>GSMPLLLDDGDPKAQTGFDLSTATTLFWRPVPVHVKQQDREDVLEELTFRILTGVAKQNHNLRILRIHISSDSDLFFLHTLEVSEEDFQSLKNDQGILVDFASFPGKIISLLEKCILAQPGDSPRFQAVLTIRGGESVFKIVEINDEKQLPHITLAFRP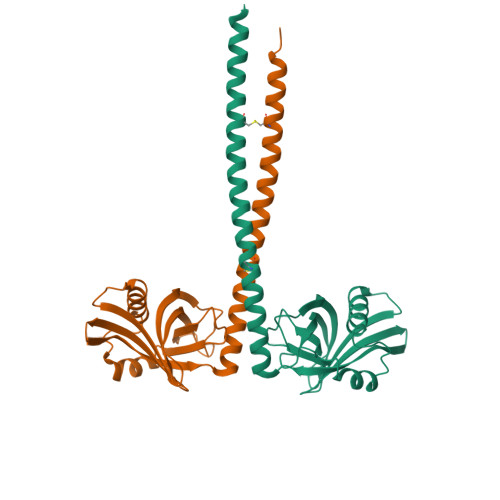GNDSVVKQFLAFRLSEVKGTCHDLSDDLSRTRDDRDSMVAQLAQCRQQLAQLREQYDKHLLEVQAQAKT[2x]>TSACENFLLPADQDGIQRQVTIFRYGQENSAPKAYLQAGLHADEFPGMLALKYLRDLLDEAARRNRIKGEIVIIPQANPIGLSQWKDGFLLGRFDHQTGTNFNRDYPDLCQLTVEKLDGQLTENAEH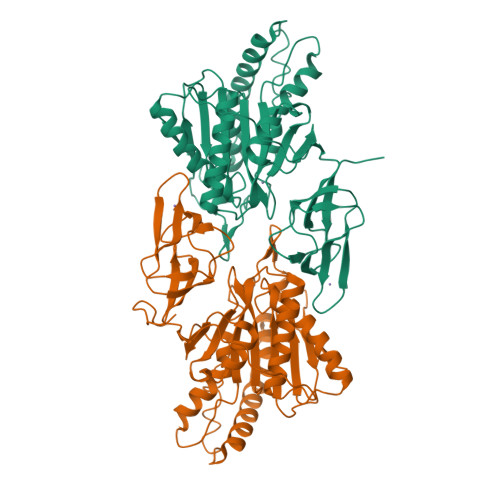NIDVIRKTMRSALSELKPEQAVDVLRHKLISESCDADLVLDLHADNQAQCHMYTLTPLWPAMHDVAAEIDARAVLLAEESGGHPFDEACSAPWMNLSRAFPDYPIPLACQSATFELGSNDEVDLRLAQDQAEALFRILIRRGFIEDVHVGELPQLACEGTLLEAMQQLKAPCQGLIVYHNRLGDFVRSGDKVVSIVDPIGETVDILAHTDGVLFARHSQTYAYPNKVIGKIAGKEPLPERKGF[4x]4-(7-chloranylquinolin-4-yl)-2-methyl-phenol | C16 H12 Cl N O | 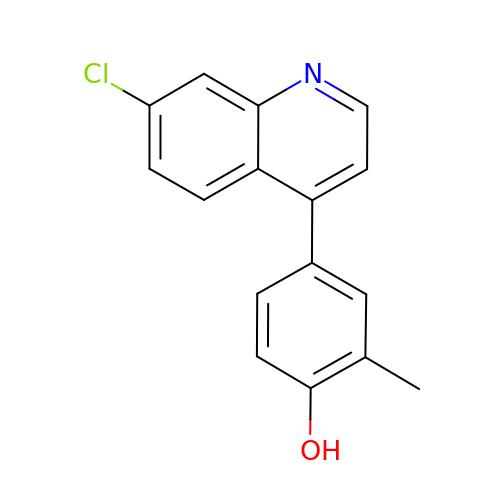VBXAMTUJCKJXCI-UHFFFAOYSA-N> TDTTLPPDDSLDRIEPVDIEQEMQRSYIDYAMSVIVGRALPEVRDGLKPVHRRVLYAMFDSGFRPDRSHAKSARSVAETMGNYHPHGDSSIYDSLVRMAQPWSLRYPLVDGQGNFGSPGNDPPAAMRYTEARLTPLAMEMLREIDEETVDFIPNYDGRVQEPTVLPSRFPNLLANGSGGIAVGMATNIPPHNLRELADAVFWALENHDADEEETLAAVMGRVKGPDFPTAGLIVGSQGTADAYKTGRGSIRMRGVVEVEEDSRGRTSLVITELPYQVNHDNFITSIAEQVRDGKLAGISNIEDQSSDRVGLRIVIEIKRDAVAKVVINNLYKHTQLQTSFGANMLAIVDGVPRTLRLDQLIRYYVDHQLDVIVRRTTYRLRKANERAHILRGLVKALDALDEVIALIRASETVDIARAGLIELLDIDEIQAQAILDMQLRRLAALERQRIIDDLAKIEAEIADLEDILAKPERQRGIVRDELAEIVDRHGDDR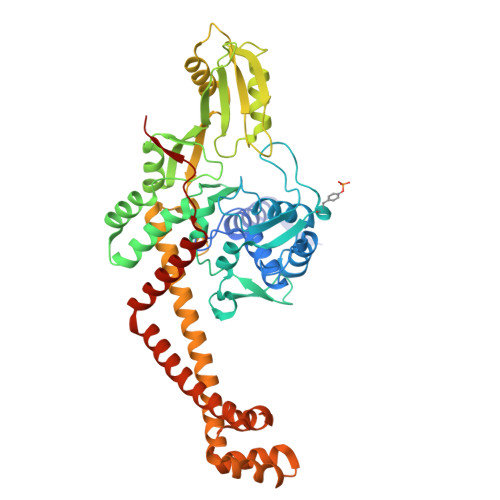RTRIIAIGSG>MSLSSEVVLMKPYEKLVERFNEMAAEFLSYFPTVKSVGNLESELDKRRFVILFRAMLRLRNEVKGYNEFDAEDLTIEEQRFADYQSKYLDMSNEFAITSEKEDAESILQDIDFELELVHRDIINVMYILALLQDLKPESSSYPKDRKAVLDTMDSNPELRSKIALIDN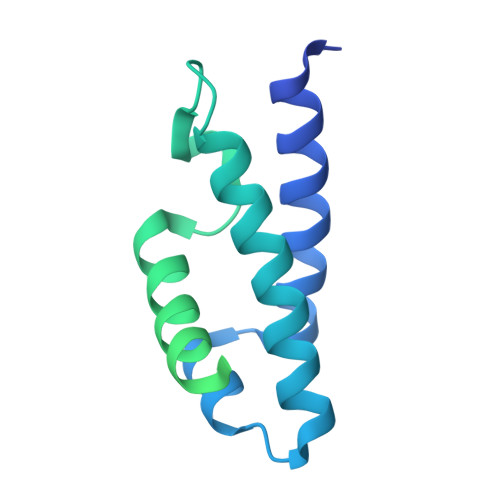FIKLHIDGRQSNDLPADMESDLDKYIATQKAIAIEQVATEEGIDSTLLHEYISEYEYLGKPKNEGHHHHHH[2x]>GNTLVVLHKSGLLEITLKTKELIRQNQATQAELDQLKEQTQMFIEATKSRAPQAWAKLQASLTS[10x];>GAMDPEFSAQLGAMQHLKDQLEQRTRMIEANIHR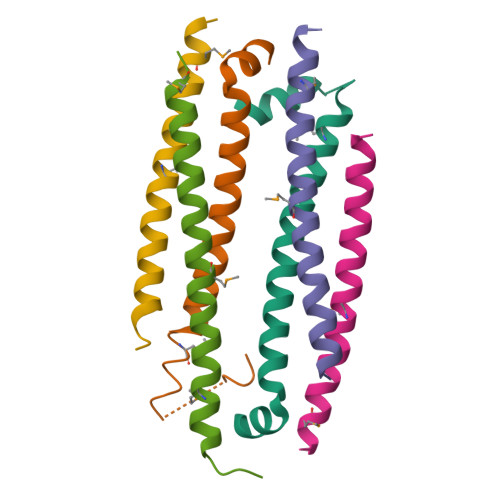QQEELRKIQEQLQMVHG[20x]> QSISPNELGLTSAQDDGPLGNEKPNYFLNFRTMNVDIFTVSHTKVDNIFGRAWYVASHDFNNGDTWRQKLTFPKEGHGMLSQFFAYFTGEINIHILYMAEQGFLRVAHTYDTEDNRKTFLSSN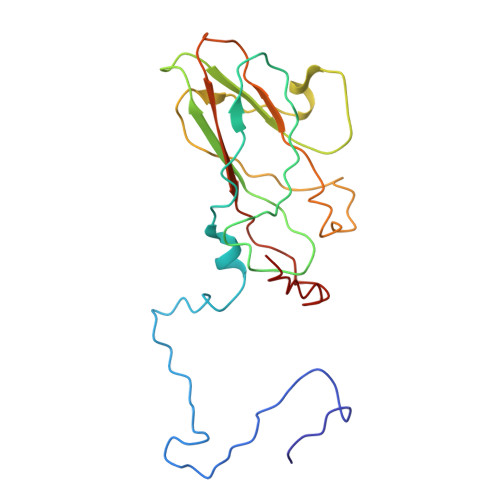GVITIPAGEQMTLSVPFYSNKPLRTVRHDSALGFLMCRPMMHGTTRTTAEVYISLRCPNFFFPVPAPKPTGSRAA> MSYRQMLIHRCDIYHEAAQAPSAGRFGIPA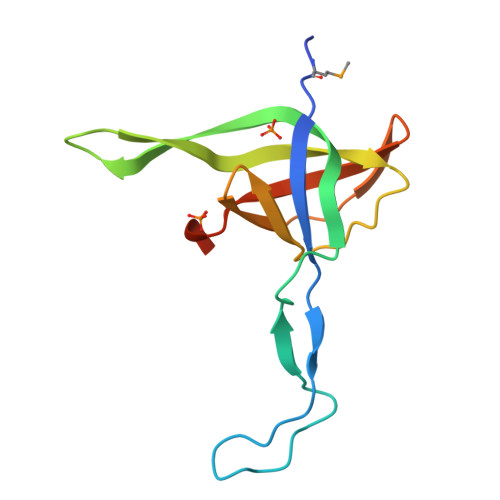DRLQPVISYPDTPDEQDVPCYFTEKTQQLIQEEPDQTVYHSFLVHFPLSADIRVNDKIIWENHKYILKLPKRIRHHHWEVVAVRDESLLEHHHHHH>[5x]MHNLQQLLPTRSLIWIFSFLTSISIWCTVAHAETEGRVQHFTGYIEDGRGIFYSLPDMKQGDIIYASMQNTGGNLDPLVGIMAEEIDPAVSLGQVLEKALASENDLISELTAVADRIFLGWDDDGGKGYSASLEFTIPRDGTYHIFAGSTITNQRLDKFQPTYTTGSFQLILGLNAPQVISGEGEPEGEVFASLASLEIKPEAHVQELEIRLDKDTRYLTQHTRNLQPGDTFHALVEPIGEAPLPRLRLTDSGGKPLAFGLIDQPGESVELNYTCDQDICELVVHVDGTDGQKDSGEAVYRLLVGINAPNLRESGQTPVGSSVFLESDLVTVGLAVDQIV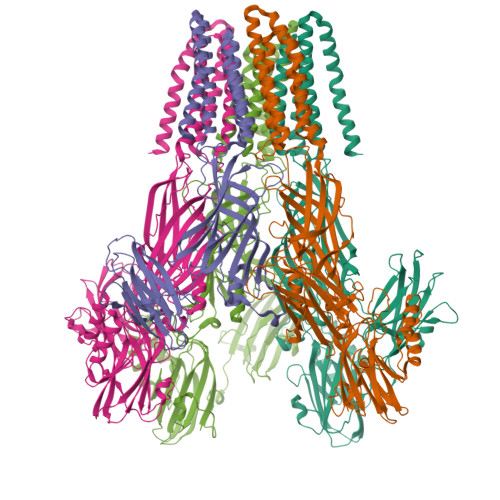GVDQRSENFSVVGTLKLSWHDPKLGFSPDQCGCTVKSFEDASIRAVAGEINLPLPSFSFYNQQGNRWSQNQVIFVTPDGRASYFERFTVTLQAPDFDFLAYPFDRQKFSIKVDLAVPTNMFIFNEIERFQQVVGDQLGEEEWVVTSYSQEITEVPFERGSTNSRFTTTLLVKRNLEYYILRIFVPLFLIISVSWVIFFLKDYGRQLEVASGNLLVFVAFNFTISGDLPRLGYLTVLDRFMIVSFCLTAIVVLISVCQKRLGAVGKQAVAAQIDTWVLVIYPLVYSLYIIWVYLRFFTDHIGW>[2x]AANDPFTIVHGNTGKCIKPVYGWIVADDCDETEDKLWKWVSQHRLFHLHSQKCLGLDITKSVNELRMFSCDSSAMLWWKCEHHSLYGAARYRLALKDGHGTAISNASDVWKKGGSEESLCDQPYHEIYTRDGNSYGRPCEFPFLIDGTWHHDCILDEDHSGPWCATTLNYEYDRKWGICLKPENGCEDNWEKNEQFGSCYQFNTQTALSWKEAYVSCQNQGADLLSINSAAELTYLKEKEGIAKIFWIGLNQLYSARGWEWSDHKPLNFLNWDPDRPSAPTIGGSSCARMDAESGLWQSFSCEAQLPYVCRKPLNNTVELTDVWTYSDTRCDAGWLPNNGFCYLLVNESNSWDKAHAKCKAFSSDLISIHSLADVEVVVTKLHNEDIKEEVWIGLKNINIPTLFQWSDGTEVTLTYWDENEPNVPYNKTPNCVSYLGELGQWKVQSCEEKLKYVCKRKGEKLNDASSDKMCPPDEGWKRHGETCYKIYEDEVPFGTNCNLTITSRFEQEYLNDLMKKYDKSLRKYFWTGLRDVDSCGEYNWATVGGRRRAVTFSNWNFLEPASPGGCVAMSTGKSVGKWEVKDCRSFKALSICKKMSHHHHHH

pmcDEC205 (CD205 or Ly75) is an endocytic receptor highly expressed on the dendritic cells with antigen-presenting function and has been widely used as a receptor target in immune therapies. DEC205 belongs to the mannose receptor family, which also includes mannose receptor (MR), PLA2R, Endo180 (8), and FcRY. MR family members are type I transmembrane proteins with a large extracellular portion, a transmembrane helix, and a short cytoplasmic region. Their ectodomains contain an N-terminal cysteine-rich domain (CysR), a fibronectin type II domain (FnII), and eight (ten for DEC205) C-type lectin-like domains (CTLDs). The functional studies of DEC205 show that it can act as a receptor for dead cells and may recognize dead cells through cellular keratins in a pH-dependent manner, as acidification usually occurs during the event of apoptosis, but the mechanism of the interaction between DEC205 and keratins remains unclear.

To investigate the structure of the CysR∼CTLD3 (residues M1- S627) fragment, we expressed the fragment in insect cells and the purified protein was applied for crystallization screening. X-ray diffraction data were collected and showed two crystal forms, one in space group C2 and the other in space group P1. The structures of the CysR∼CTLD3 fragment show a C-shaped conformation in both crystal forms and they are quite similar with the r.m.s. deviation of Cα atoms of 0.89 Å. In P1 crystals, a homodimer of the fragment forms in one asymmetric unit, where the dimeric interface is contributed by the interactions of CysR∼CTLD1 and CTLD3. The CysR∼CTLD2 region of DEC205 has an L-shaped conformation that is also found in the crystal structures of MR and Endo180 and the C-shaped conformation of the CysR∼CTLD3 fragment of DEC205 is similar to that of MR at acidic condition. Notably, the structure of the CLTD3 of DEC205 is different from the conventional CTLD fold with two unique loop regions (loop 1 and loop 2). Loop 1 (residue E521-C528) replaces a conserved α-helix in the conventional CTLDs, and loop 2 (residue T573-A592) becomes much longer and partially missing in the crystal structure. In addition, previous reports have shown that oligomerization could be a common feature for the MR family members which may correlate with ligand recognition. Recent cryoEM data also suggest that DEC205 may form dimers or tetramers, which might be relevant to CpG binding. Similarly, the dimerization or oligomerization of DEC205 may also promote the binding of keratins.>GSGSRMKTVDKSKTLTKFEEFFSLQDYKDRVFEAIEKYPNVRSIEVDYLDLEMFDPDLADLLIEKPDDVIRAAQQAIRNIDRLRKNVDLNIRFSGISNVIPLRELRSKFIGKFVAVDGIVRKTDEIRPRIVKAVFECRGCMRHHAVTQSTNMITEPSLCSECGGRSFRLLQDESEFLDTQTLKLQEPLENLSGGEQPRQITVVLEDDLVDTLTPGDIVRVTGTLRTVRDERTKRFKNFIYGNYTEFLEQEFEELQISEEDEEKIKE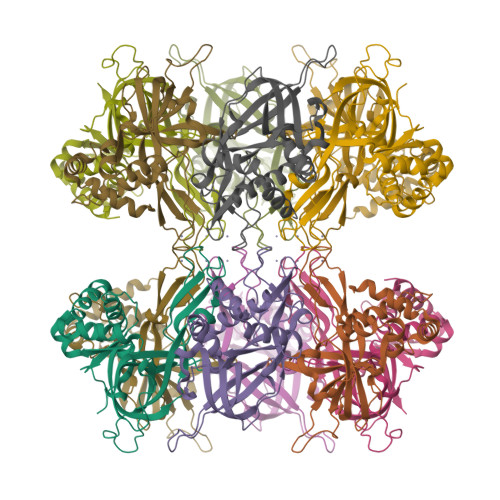LAGDPNIYEKIIR[6x]>[2x]MRAVVMRARGGPEVLEVADLPVPEPGPKEVRVRLKAAALNHLDVWVRKGVASPKLPLPHVLGADGSGVVDAVGPGVEGFAPGDEVVINPGLSCGRCERCLAGEDNLCPRYQILGEHRHGTYAEYVVLPEANLAPKPKNLSFEEAA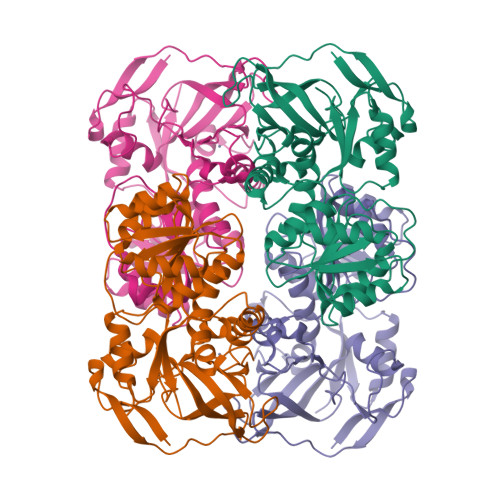AIPLTFLTAWQMVVDKLGVRPGDDVLVMAAGSGVSVAAIQIAKLFGARVIATAGSEDKLRRAKALGADETVNYTHPDWPKEVRRLTGGKGADKVVDHTGALYFEGVIKATANGGRIAIAGASSGYEGTLPFAHVFYRQLSILGSTMASKSRLFPILRFVEEGKLKPVVGQVLPLEAAAEGHRLLEERRVFGKVVLQVG> UXCUCCUAGUACGAGAGGACCGGAGUG

When deamination affects guanosines, a xanthosine (X) containing RNA is generated. Applying NMR spectroscopy and X-ray crystallography, we demonstrate that X can form distinct wobble geometries with uridine depending on the sequence context. In contrast, X pairing with cytidine occurs either through wobble geometry involving protonated C or in Watson–Crick-like arrangement. We therefore utilized the 27 nt fragment of the E. coli 23S rRNA sarcin−ricin loop (SRL), the 12 nt RNA 5′-CGCGAAUUACGC, and the 14 nt RNA 5′-GGUAUUGCGGUACC, all of them are known crystallization scaffolds.

X-ray structure determination showed that the X nucleobases are well-defined in the electron density maps. For the SRL RNA structure (solved at 0.9 Å resolution), X2648 pairs with U2672 in wobble geometry (w1U–X) forming X-N1H•••O2-U and X-O6•••HN3-U hydrogen bonds similar to a typical wobble G–U pair. Characteristically, a water molecule bridges the O2 of X2648 and the 2′-OH of U2672. Of note, the unmodified RNA scaffold contains a G–U wobble pair at the very position (2648–2672). Superimpositions of the X-modified RNA structure with the unmodified RNA showed a root-mean-square deviation (rmsd) of 0.10 Å (within the errors on coordinates of 0.10 Å). Finally we mention that all our attempts to crystallize the SRL scaffold with a replacement of individual A–U or G–C pairs (at diverse positions) by X–U or X–C failed.> GSNNVLPTWSLDSNGEMRSRLSLSEVLDSGDLMKFAVDKTGCQFLEKAVKGSLTSYQKFQLFEQVIGRKDDFLKLSTNIFGNYLVQSVIGISLATNDDGYTKRQEKLKNFISSQMTDMCL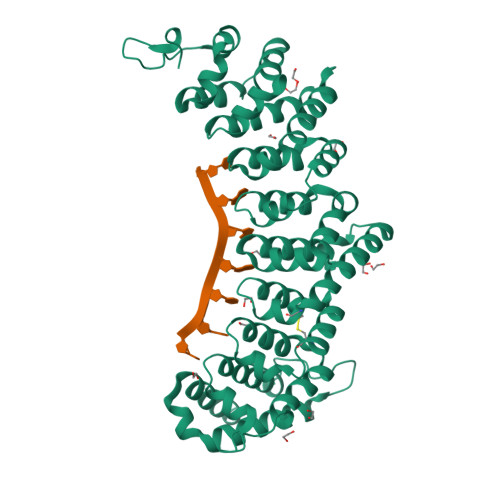DKFACRVIQSSLQNMDLSLACKLVQALPRDARLIAICVDQNANHVIQKVVAVIPLKNWEFIVDFVATPEHLRQICSDKYGSYVVSTIIEKLTADSMNVDLTSAAQNLRERALQRLMTSVTNRCQELATNEYANYIIQHIVSNDDLAVYRECIIEKCLMRNLLSLSQEKFASHVVEKAFLHAPLELLAEMMDEIFDGYIPHPDTGKDALDIMMFHQFGNYVVQCMLTICCDAVSGRRQTKEGGYDHAISFQDWLKKLHSRVTKERHRLSRFSSGKKMIETLANLRSTHPIYELQ>MASQVGAINSVNALISRVFVQPKGDLADRLNSRVTVVILAVSSALLLSSHFIGDPITCWTPAQFNAQWVNFVNQYCFVHGTYFVPLDQQLAFEEEERTKVSIQYYQWVPYVFALQAFLFYIPRFIWKAMIAYSGYDLAAAVKYVDRFWSENRDKDDKFKTRLAAFEGRPSVYIWDGIRLARKKRSRNMALFYTLSTVWQAVNAWIQFYILTQLLDSSIYTLWGPSILGDLLQGNDWQTTGHFPRIVHCDFNRRRPASVQLDTV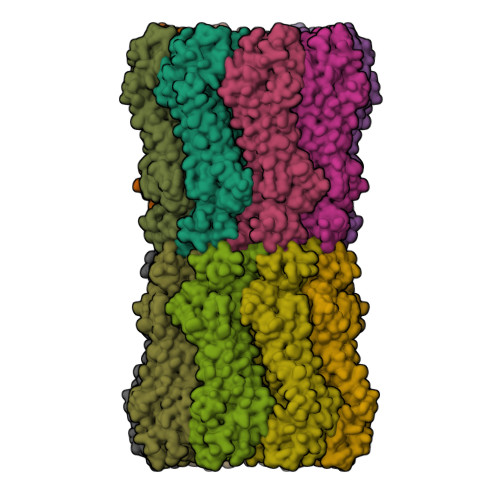LCVLTLNIYYEKLFIFLWFWLVFVAVVSTVNCFKWIYYLCNKTKAQKTIKNYLSTAPIKSTISDDQFFSALGEDGLFIMDQMALNLGDIPASYLTISMRNICQDFIESEDYIDEERTPFVKSIKHT[16x]> APDWVPPEVFDLVAEDKARCMSEHGTTQAQIDDVDKGNLVNEPSITCYMYCLLEAFSLVDDEANVDEDIMLGLLPDQLQERAQSVMGKCLPTSGSDNCNKIYNLA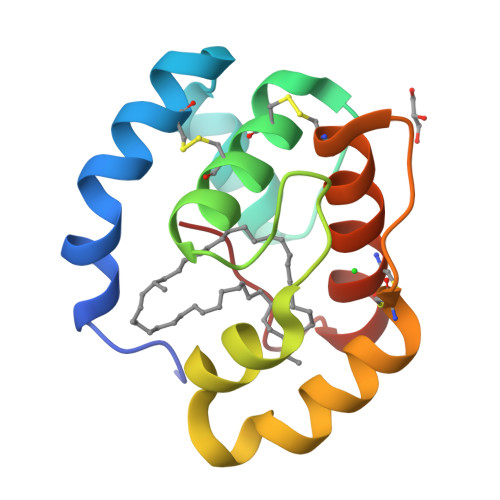KCVQESAPDVWFVI N-carboxy-L-phenylalanyl-N-{(2S,3R)-3-hydroxy-4-methoxy-4-oxo-1-[(3R)-2-oxo-3,4-dihydro-2H-pyrrol-3-yl]butan-2-yl}-L-lysinamide 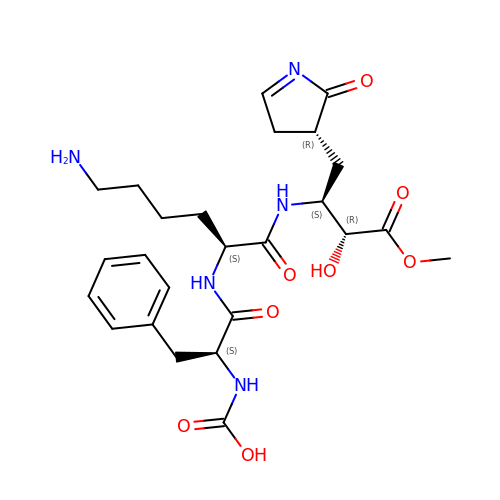| C25 H35 N5 O8 | WFSLHCGPTMFRHH-VYJAJWGXSA-N>[4x]SEFLPTMEGPPTFNPPVPYFGRL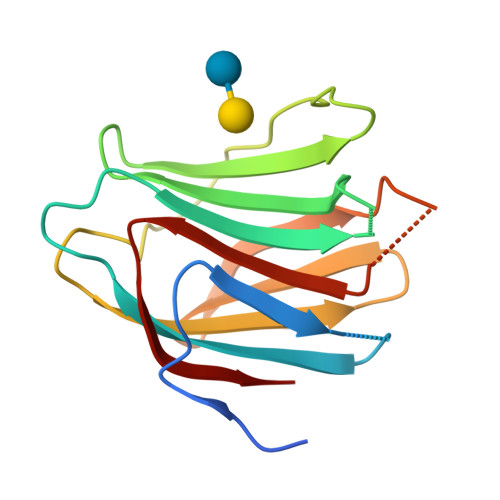QGGLTARRTIIIKGYVPPTGKSFAINFKVGSSGDIALHINPRMGNGTVVRNSLLNGSWGSEEKKITHNPFGPGQFFDLSIRCGLDRFKVYANGQHLFDFAHRLSAFQRVDTLEIQGDVTLSYVQI> SDSLSKSPENWMSKLDDGKHLTEINIPGSHDSGSFTLKDPVKSVWAKTQDKDYLTQMKSGVRFFDIRGRASADNMISVHHGMVYLHHELGKFLDDAKYYLSAYPNETIVMSMKKDYDSDSKVTKTFEEIFREYYYNNPQYQNLFYTGSNANPTLKETKGKIVLFNRMGGTYI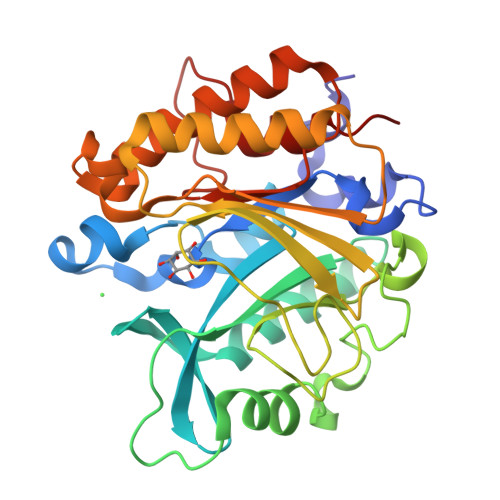KSGYGADTSGIQWADNATFETKINNGSLNLKVQDEYKDYYDKKVEAVKNLLAKAKTDSNKDNVYVNFLSVASGGSAFNSTYNYASHINPEIAKTIKANGKARTGWLIVDYAGYTWPGYDDIVSEIIDSNKL>RMSDGAAPKANGSEASGQDLVPAAVEQAVPIQPVAGAALAAPAAGQINQIDPWIFQNFVQCPLGEFSISPRNTPGEILFDLALGPGLNPYLAHLSAMYTGWVGNMEVQLVLAGNAFTAGKVVVALVPPYFPKGSLTTAQITCFPHVMCDVRTLEPIQLPLLDVRRVLWHATQDQEESMRLVCMLYTPLRTNSPGDESFVVSGRLLSKPAADFNFVYLTPPIERTIYRMVDLPVIQPRLCTHARWPAPVYGLLVDPSLPSNPQWQNGRVHVDGTLLGTTPISGSWVSCFAAEAAYEFQSGTGEVATFTLIEQDGSAYVPGDRAAPLGYPDFSGQLEIEIQTETTKTGDKLKVTTFEMILGP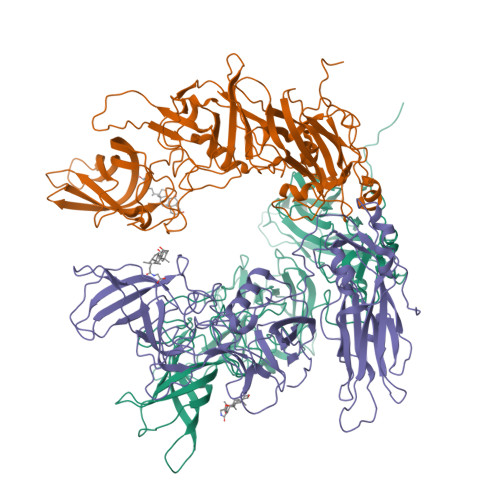TTNADQAPYQGRVFASVTAAASLDLVDGRVRAVPRSIYGFQDTIPEYNDGLLVPLAPPIGPFLPGEVLLRFRTYMRQIDTADAAAEAIDCALPQEFVSWFASNAFTVQSEALLLRYRNTLTGQLLFECKLYNEGYIALSYSGSGPLTFPTDGIFEVVSWVPRLYQLASVGSLATGRMLKQ[3x]>[3x]MTMQIKIKYLDETQTRISKIEQGDWIDLRAAEDVTIKKDEFKLVPLGVAMELPEGYEAHVVPRSSTYKN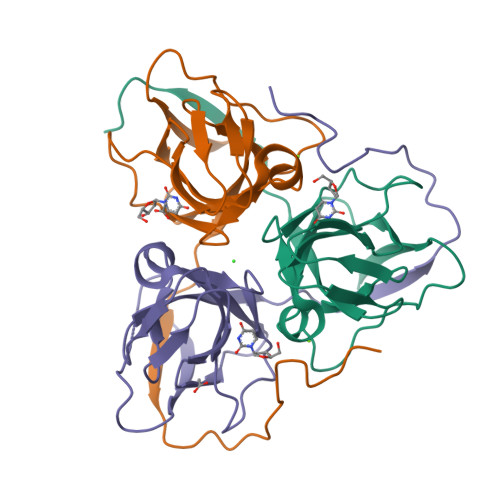FGVIQTNSMGVIDESYKGDNDFWFFPAYALRDTEIKKGDRICQFRIMKKMPAVELVEVEHLGNEDRGGLGSTGTK> GSMAAG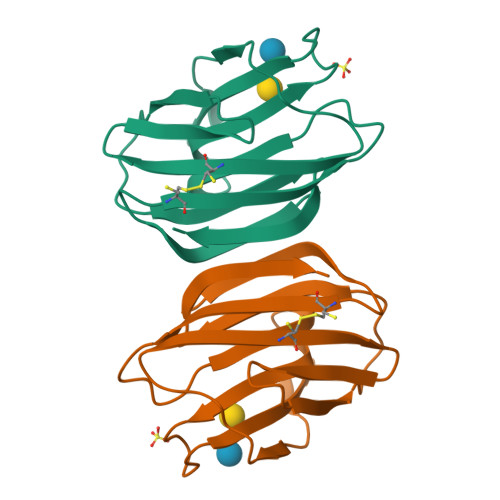MVMNNFSLKQGHCLELKGFIPKDAKSFAINLGKDSSNYVIHFNPRFDHEGDTNKIICNSKEENSWGTEQRENVFPFQQGAETSICFEYQADHLKVKLSDGQEFNFPIRMPLDTITFLSMDGIELKAISLH>MEKGTPPTHDSDNWMGRAKEIGNGGWDQFQFLFFDPNGYLYAVSNDKLYKASPPQSDTDNWIARATEIGSGGWSGFKFLFFHPNGYLYAVRGQRFYKA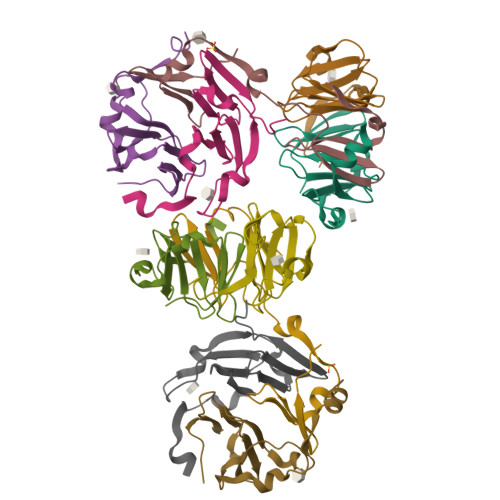LPPVSNQD[10x]>[4x]MIQITVIQID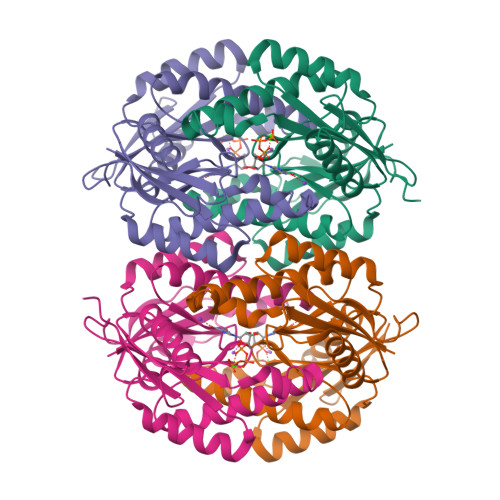NYGPWTVTPNPRRESDLQALQSRLYADLNLMFGAHKGLVFYTRFDNLIAITNGIDLITHKRIQESIRNRYPFTVSMVIASAETPYEAQKLATETLQEYGSAQDENRKEVLDVANELVVDGYVQIAHIDINNITGTLTDIVSAYDTYLNVNKVKLALMEELLKYNALLFFIGGDNFMAPSNGMSEEDFLDIFNRINKKYKIELKAGIGIGRTAEDASNLADIGLEKIRGKLVDKNVCTLKQDDFLESKMGMGKIYHPQF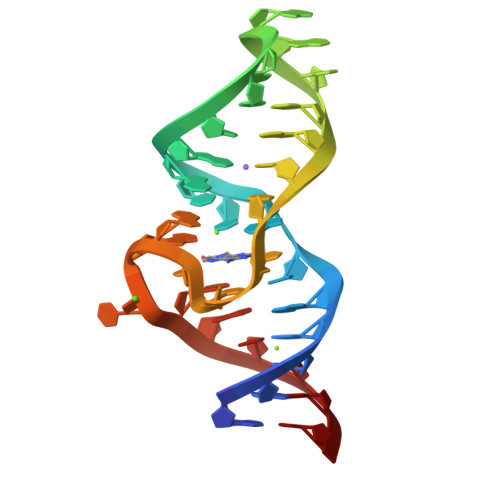>GGCGAUACCAGCCGAAAGGCCCUUGGCAGCGCC[4x]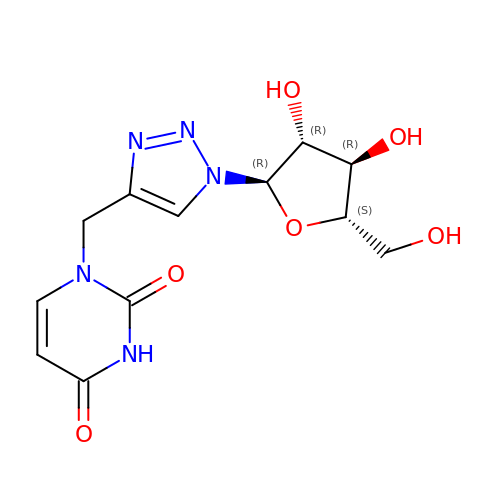1-{[1-(alpha-L-arabinofuranosyl)-1H-1,2,3-triazol-4-yl]methyl}-2,4-dioxo-1,2,3,4-tetrahydropyrimidine | C12 H15 N5 O6 | HUSMKQOXUIOPRU-CPOMMVLXSA-N>[16x]XQADLF;>[16x]HMHFTIQREALLKPLQLVAGVVERRQTLPVL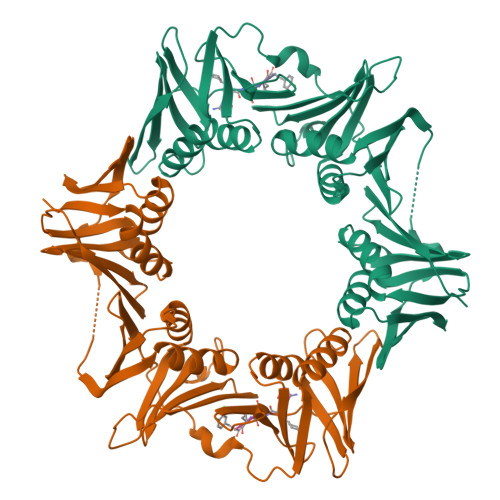SNVLLVVEGQQLSLTGTDLEVELVGRVVLEDAAEPGEITVPARKLMDICKSLPNDVLIDIRVEEQKLLVKAGRSRFTLSTLPANDFPTVEEGPGSLNFSIAQSKLRRLIDRTSFAMAQQDVRYYLNGMLLEVNGGTLRSVATDGHRLAMCSLDAQIPSQDRHQVIVPRKGILELARLLTEQDGEVGIVLGQHHIRATTGEFTFTSKLVDGKFPDYERVLPRGGDKLVVGDRQQLREAFSRTAILSNEKYRGIRLQLSNGLLKIQANNPEQEEAEEEVQVEYNGGNLEIGFNVSYLLDVLGVIGTEQVRFILSDSNSSALVHEADNDDSAYVVMPMRL>MAKKDEKSHKNAPLIGIDIGGTGIKGGIVDLKKGKLLGERFRVPTPQPATPESVAEAVALVVAELSARPEAPAAGSPVGVTFPGIIQHGVVHSAANVDKSWLNTDIDALLTARLGRPVEVINDADAAGLAEARYGAGAGVKGTVLVITLGTGIGSAFIFDGKLVPNAELGHLEIDGHDAETKASAVARERDGLSWDEYSVLLQRYFSHVEFLFSPELFIVGGG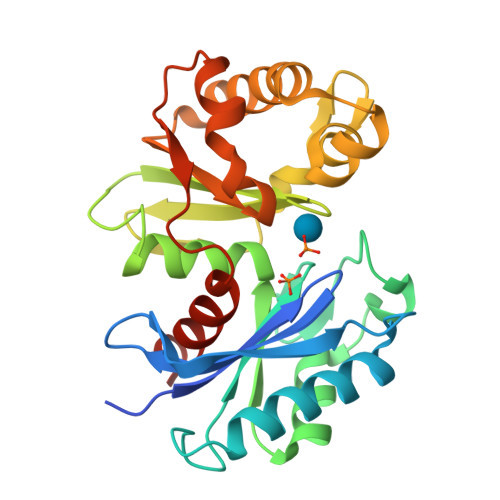ISKRADEYLPNLRLRTPIVPAVLRNEAGIVGAAIEIALQHKLAK[2x]> MAMHPRKDWYELTRATNWTPSYVTEEQLFPERMSGHMGIPLEKWESYDEPYKTSYPEYVSIQREKDAGAYSVKAALERAKIYENSDPGWISTLKSHYGAIAVGEYAAVTGEGRMARFSKAPGNRNMATFGMMDELRHGQLQLFFPHEYCKKDRQFDWAWRAYHSNEWAAIAAKHFFDDIITGRDAISVAIMLTFSFETGFANM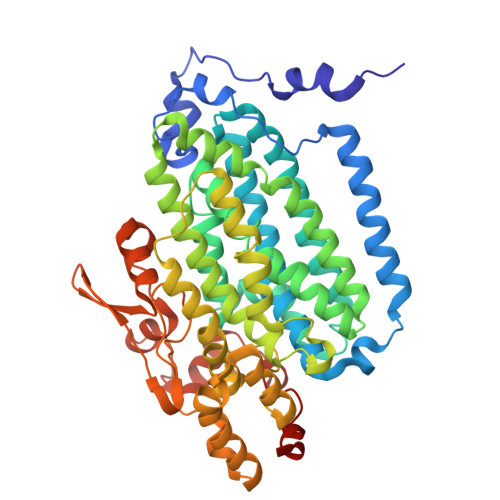QFLGLAADAAEAGDYTFANLISSIQTDESRHAQQGGPALQLLIENGKREEAQKKVDMAIWRAWRLFAVLTGPVMDYYTPLEDRSQSFKEFMYEWIIGQFERSLIDLGLDKPWYWDLFLKDIDELHHSYHMGVWYWRTTAWWNPAAGVTPEERDWLEEKYPGWNKRWGRCWDVITENVLNDRMDLVSPETLPSVCNMSQIPLVGVPGDDWNIEVFSLEHNGRLYHFGSEVDRWVFQQDPVQYQNHMNIVDRFLAGQIQPMTLEGALKYMGFQSIEEMGKDAHDFAWADKCKPAMKKSA> MSFESKKPMRTWSHLAEMRKKPSEYDIVSRKLHYSTNNPDSPWELSPDSPMNLWYKQYRNASPLKHDNWDAFTDPDQLVYRTYNLMQDGQESYVQS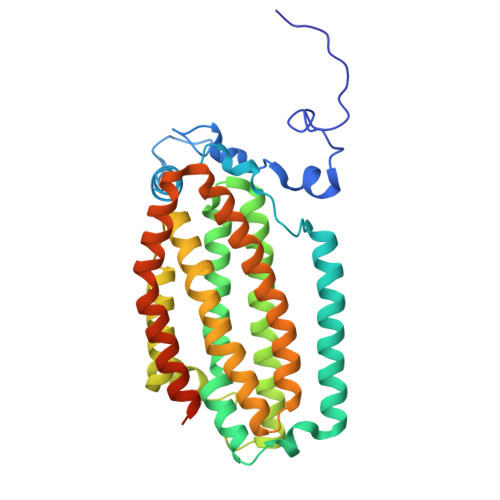LFDQFNEREHDQMVREGWEHTMARCYSPLRYLFHCLQMSSAYVQQMAPASTISNCCILQTADSLRWLTHTAYRTHELSLTYPDAGLGEHERELWEKEPGWQGLRELMEKQLTAFDWGEAFVSLNLVVKPMIVESIFKPLQQQAWENNDTLLPLLIDSQLKDAERHSRWSKALVKHALENPDNHAVIEGWIEKWRPLADRAAEAYLSMLSSDILHAQYLERSTSLRASILTV> AVSLDRTRAVFDGSEKSMTLDISNDNKQLPYLAQAWIENENQEKIITGPVIATPPVQRLEPGAKSMVRLSTTPDISKLPQDRESLFYFNLREIPPRSEKANVLQIALQTKIKLFYRPAAIKTRPNEVWQDQLILNKVSGGYRIENPTPYYVTVIGLGGSEKQAEEGEFETVMLSPRSEQTVKSANYNTPYLSYINDYGGRPVLSFICNGSRCSVKKEK;> DVQINIRNNVYIPPCTINNGQNIVVDFGNINPEHVDNSRGEVTKTISI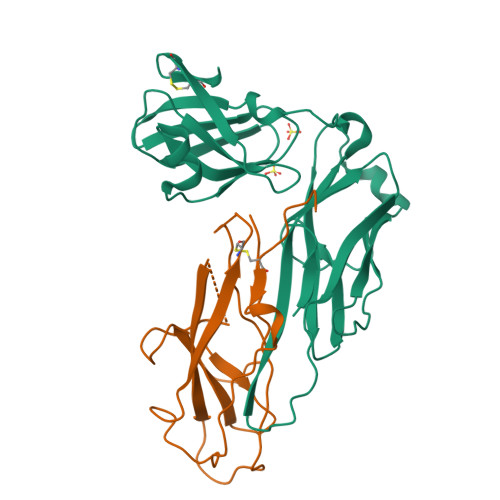SCPYKSGSLWIKVTGNTMGGGQNNVLATNITHFGIALYQGKGMSTPLTLGNGSGNGYRVTAGLDTARSTFTFTSVPFRNGSGILNGGDFRTTASMSMIYN>[2x]GNSDDARTSIEQRSNAVSQVLLGIFSYV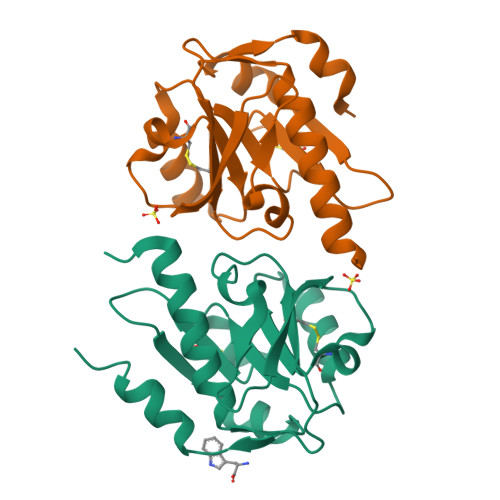RWPKEPAVLQLCVVGPTEYADGLLRGMVQANGRRVHAERRAVDNPDLGTLCNVIYLGVVDERERQQVFRSLAGHPVLSISERGTECSVGSMFCLNVGGPRITFEANLDSIARSGVRVHPSVLKLARRQATP> MNDDRETPPKRKPGEDDTLFDIDFLDDTTSHSGSRSKVTNSHANANYI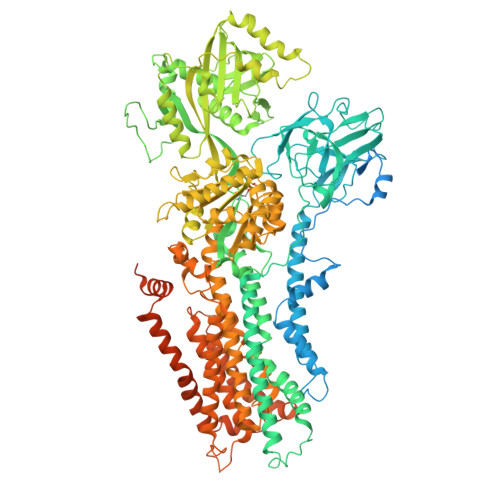PPSHVLPEETIDLDADDDNIENDVHENLFMSNNHDDQTSWNANRFDSDAYQPQSLRAVKPPGLFARFGNGLKNAFTFKRKKGPESFEMNHYNAVTNNELDDNYLDSRNKFNIKILFNRYILRKNVGDAEGNGEPRVIHINDSLANSSFGYSDNHISTTKYNFATFLPKFLFQEFSKYANLFFLCTSAIQQVPHVSPTNRYTTIGTLLVVLIVSAMKECIEDIKRANSDKELNNSTAEIFSEAHDDFVEKRWIDIRVGDIIRVKSEEPIPADTIILSSSEPEGLCYIETANLDGETNLKIKQSRVETAKFIDVKTLKNMNGKVVSEQPNSSLYTYEGTMTLNDRQIPLSPDQMILRGATLRNTAWIFGLVIFTGHETKLLRNATATPIKRTAVEKIINRQIIALFTVLIVLILISSIGNVIMSTADAKHLSYLYLEGTNKAGLFFKDFLTFWILFSNLVPISLFVTVELIKYYQAFMIGSDLDLYYEKTDTPTVVRTSSLVEELGQIEYIFSDKTGTLTRNIMEFKSCSIAGHCYIDKIPEDKTATVEDGIEVGYRKFDDLKKKLNDPSDEDSPIINDFLTLLATCHTVIPEFQSDGSIKYQAASPDEGALVQGGADLGYKFIIRKPNSVTVLLEETGEEKEYQLLNICEFNSTRKRMSAIFRFPDGSIKLFCKGADTVILERLDDEANQYVEATMRHLEDYASEGLRTLCLAMRDISEGEYEEWNSIYNEAATTLDNRAEKLDEAANLIEKNLILIGATAIEDKLQDGVPETIHTLQEAGIKIWVLTGDRQETAINIGMSCRLLSEDMNLLIINEETRDDTERNLLEKINALNEHQLSTHDMNTLALVIDGKSLGFALEPELEDYLLTVAKLCKAVICCRVSPLQKALVVKMVKRKSSSLLLAIGDGANDVSMIQAAHVGVGISGMEGMQAARSADIAVGQFKFLKKLLLVHGSWSYQRISVAILYSFYKNTALYMTQFWYVFANAFSGQSIMESWTMSFYNLFFTVWPPFVIGVFDQFVSSRLLERYPQLYKLGQKGQFFSVYIFWGWIINGFFHSAIVFIGTILIYRYGFALNMHGELADHWSWGVTVYTTSVIIVLGKAALVTNQWTKFTLIAIPGSLLFWLIFFPIYASIFPHANISREYYGVVKHTYGSGVFWLTLIVLPIFALVRDFLWKYYKRMYEPETYHVIQEMQKYNISDSRPHVQQFQNAIRKVRQVQRMKKQRGFAFSQAEEGGQEKIVRMYDTTQKRGKYGELQDASANPFNDNNGLGSNDFESAEPFIENPFADGNQNSNRFSSSRDDISFDI> ER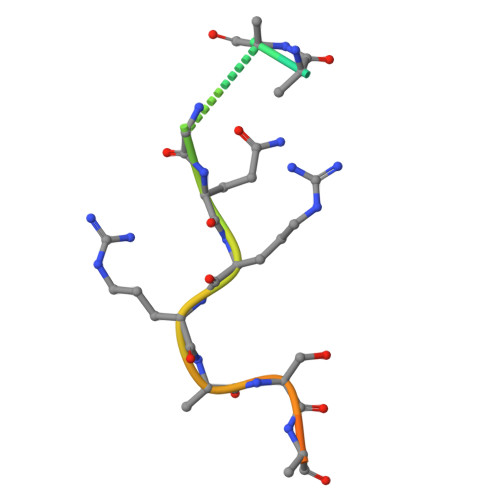PRRRSRGQRRRSNRRERQ>[2x]QSMPEDLDALLDLAARHGLDLDGGTLRTEEIGLDFRVAFARAHDGGDWVLRLPRRPDVLERAAVEGRLLAMLAPHLDVAVPDWRISTSELIAYPLLPGSPGLTVAADGEVSWHVDMASTVYARSLG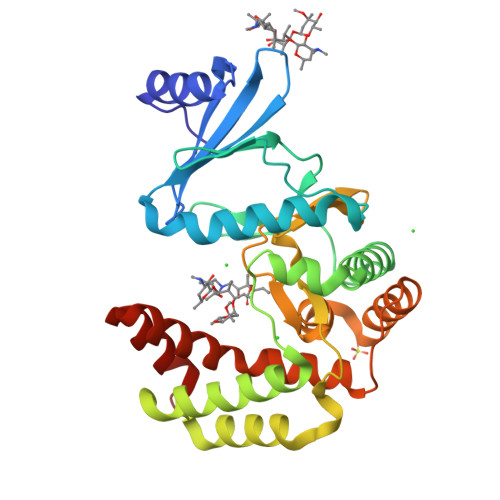SVVAQLHAVDAEAAAATGIEVRSPAQVRGAWRQDLARVGAEFEIAPALRERWEAWLADDGCWPGHSVLTHGELYPAHTLVEDERITAVLDWTTAAVGDPAKDLMFHQVSAPSAIFEVALQAYAEGGGRPWPGLARHCTEMFSAAPLGYGLYALATGEAAHREAAAAALNPPEER>SNAVDSLLDSVKWDNKGLAVAIAQNVDTGAILMQGFANREAVATTISSRKATFYSRSRSSLWTKGETSNNFINVHDVFLDCDRDSIIYLGKPDGPTCHTGAETCYYTPVFDLLKEEEVEGNKLALTSLYALESTISQRKA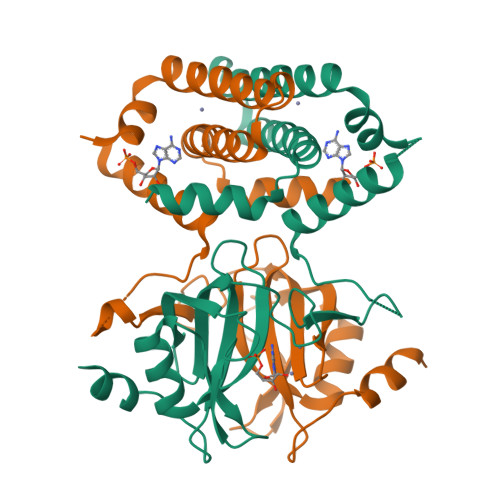EVVEENGKPSWTKRLLLNDKLLCSKIREEANELCETLENNEDKSRTASEMADVLYHAMVLLALKDVKVEEVLQVLRQRFSKSGIEEKRSRPTQKSVEN[6x]> XEVKQLEAEVEELESELWHLENEVARLEKENAE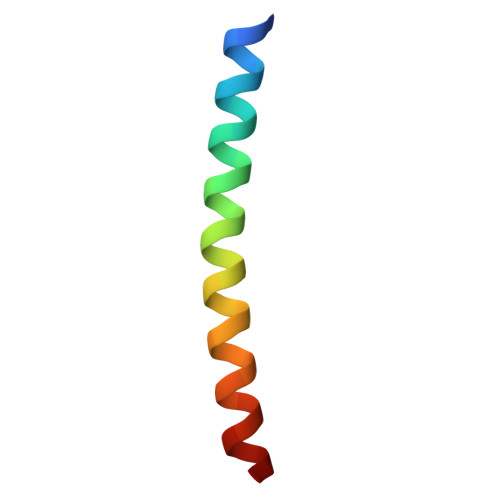CEA>GASRTERLLNLLLALLNTKVGLPRAVLREKVYHDSADNDVAFGRMFERDKVDLKQFGFEIETLMDPRNFGADDPASARYRIGKDSNRLPDVSLTPAESTVLLLAAQLWERAALGSAAANAVRKLQAAGGFRDVDLPAGVQPRIKPAGQAFDDVVAAMHGKHPIRFGYQAVSTGREEVREVEPWGLGSRFGQWYLVGLDRGRGAKRVFRLSRMTTAISVLTTGSFHPPKDFNARAELDELNELPVRQATLVIDKDKLLALRKKATSLQDAPDESGRDRITVDFRDPEQLAEELASYGPHVKVTGPAELSAAVVRRLQAAADFDDAPLPPLEFPEAGRAPRARKRTSEDQLARMLQLVPFLVHHQGLHIQEVADHFGISRKALIDDLKILICSGLPEGYPDDLLDIQWENDHVYISEHLDLNRPVRFSEEEAAALLTGLAMLGDLPALAGVPEDGSGSALESVTIKLTGAAGEAARLAGSVSGQSVAPEQAQAFAAITQAIREGRQLRLRYFSLQRDEVTERDVDPLRLYSLDSTWYFEAYCHSKAGVRNFRLDRVESLEPNGRAVSGSATAGQDFPARLFTPGEDDVLVCLELTRQGAGLADDYYAERTAPLPDGGLLAEVRFGDAGWLPMFVSQHGGSVRILEPESLRQETRAWIDAALVQYDS[2x]

During the mycobacterial DNA damage response, the heterodimeric transcriptional regulator PafBC activates most of the genes required for an adequate response to DNA stress. Based on sequence similarity, PafBC belongs to a family of bacterial regulators featuring a winged helix-turn-helix (HTH) domain at the N-terminus, followed by a C-terminal domain of unknown function named WYL domain after a consecutive W-Y-L sequence motif. PafBC activates its target genes via a promoter motif called RecA-NDp (RecA-independent promoter), which was demonstrated by in vivo identification of PafBC binding sites using cell culture cross-linking followed by immunoprecipitation of PafBC-DNA complexes. Mycobacteria and many other actinobacteria employ two distinct yet interconnected pathways in order to upregulate the expression of specific sets of genes required for repair and survival of DNA damage.

In this study, we determine the crystal structure of PafBC from Arthrobacter aurescens in its non-activated, DNA-free state. Three-dimensional crystals suitable for data collection were ultimately obtained using an A. aurescens PafBC construct (AauPafBCΔNC), which was shortened by 17 amino acids at the N-terminus and 7 amino acids at the C-terminus based on sequence alignment, since these residues are not conserved amongst the orthologs and not even present in most of them. AauPafBCΔNC crystallized in space group P212121 with two molecules in the asymmetric unit, and the structure was refined to 2.2 Å with an Rwork/Rfree of 20%/24%. The PafBC structure features six distinct domains, three in each of the homologous PafB and PafC modules. The structure reveals that the WYL domain exhibits an Sm-fold, commonly encountered in RNA-binding proteins, and is followed by an additional C-terminal extension (WCX) domain featuring a ferredoxin-like fold. The HTH domain of PafB (HTH-B) is accessible in the structure, since only helix H1 and a small part of H3 make hydrophobic contacts to the rest of the molecule. Importantly, the putative recognition helix (H3) appears wedged into the protein core, and following H3, a long loop extends around the back of the central α-helix of PafB (α4) and the WYL-B domain. The PafBC WYL domains are located at the periphery of the molecule on opposite sides, while the WCX domains come together to form a dimeric interaction module. We obtained the crystal structure of PafBC in the absence of DNA, in a largely asymmetric domain arrangement that is likely characteristic for the non-activated state.> FMVSLPRMVYPQPKVLTPCRKDVLVVTPWLAPIVWEGTFNIDILNEQFRLQNTTIGLTVFAIKKYVAFLKLFLETAEKHFMVGHRVHYYVFTDQPAAVPRVTLGTGRQLSVLEVRAYKRWQDVSMRRMEMISDFCERRFLSEVDYLVCVDVDM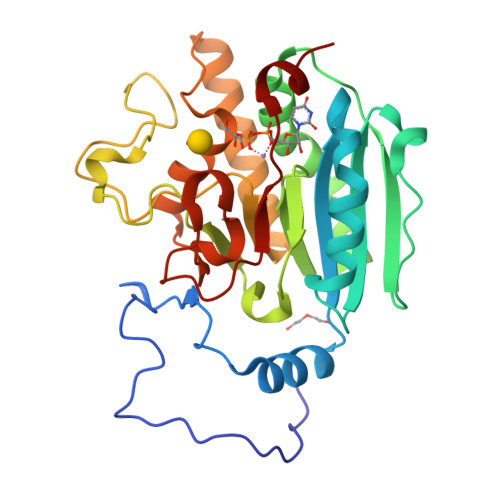EFRDHVGVEILTPLFGTLHPSFYGSSREAFTYERRPQSQAYIPKDEGDFYYMGAFFGGSVQEVQRLTRACHQAMMVDQANGIEAVWHDESHLNKYLLRHKPTKVLSPEYLWDQQLLGWPAVLRKLRFTAVPKNHQAVRNP>[2x]MSNKCDVVVVGGGISGMAAAKLLHDSGLNVVVLEARDRVGGRTYTLRNQKVKYVDLGGSYVGPTQNRILRLAKELGLETYKVNEVERLIHHVKGKSYPFRGPFPPVWNPITYLDHNNFWRTMDDMGREIPSDAPWKAPLAEEWDNMTMKELLDKLCWTESAKQLATLFVNLCVTAETHEVSALWFLWYVKQCGGTTRIISTTNGG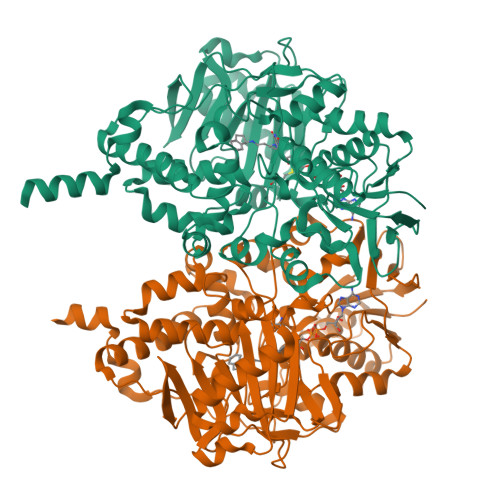QERKFVGGSGQVSERIMDLLGDRVKLERPVIYIDQTRENVLVETLNHEMYEAKYVISAIPPTLGMKIHFNPPLPMMRNQMITRVPLGSVIKCIVYYKEPFWRKKDYCGTMIIDGEEAPVAYTLDDTKPEGNYAAIMGFILAHKARKLARLTKEERLKKLCELYAKVLGSLEALEPVHYEEKNWCEEQYSGGCYTTYFPPGILTQYGRVLRQPVDRIYFAGTETATHWSGHMEGAVEAGERAAREILHAMGKIPEDEIWQSEPESVDVPAQPITTTFLERHLPSVPGLLRLIGLTTIFSATALGFLAHKRGLLVRV>GAKQVDVHDPVMTREGDTWYLFSTGPGITIYSSKDRVNWRYSDRAFATEPTWAKRVSPSFDGHLWAPDIYQHKGLFYLYYSVSAFGKNTSAIGVTVNKTLNPASPDYRWEDKGIVIESVPQRDLWNAIAPAIIA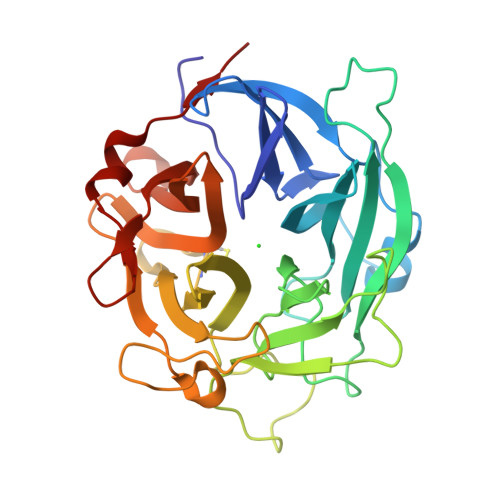DDHGQVWMSFGSFWGGLKLFKLNDDLTRPAEPQEWHSIAKLERSVLMDDSQAGSAQIEAPFILRKGDYYYLFASWGLCCRKGDSTYHLVVGRSKQVTGPYLDKTGRDMNQGGGSLLIKGNKRWVGLGHNSAYTWDGKDYLVLHAYEAADNYLQKLKILNLHWDGEGWPQVDEKELDSYISQRLK[6x]Transcription activator-like (TAL) effectors specifically bind to double stranded (ds) DNA through a central domain of tandem repeats. Each TAL effector (TALE) repeat comprises 33–35 amino acids and recognizes one specific DNA base through a highly variable residue at a fixed position in the repeat. The crystal structures of TAL effector (TALE) proteins bound to their respective target DNAs have revealed that the residue at position 13 is the only one directly involved in DNA base recognition, whereas the 12th residue stabilizes the proper loop conformation. dHax3, an engineered TALE protein, proved to be a useful scaffold for structural characterizations. We then present fifteen crystal structures of engineered dHax3 variants in complex with target DNA molecules, which elucidate the structural basis for the recognition of bases adenine (A) and guanine (G) by reported or uncharacterized TALE codes.

The structural observation suggests that Ile34 may not be a major contributor to the affinity of DNA binding by TALE repeats, consistent with the classification of NI as a “weak” TALE code. It also insinuates that base A may “tolerate” a wide range of amino acids at position 34 of a TALE repeat when there is no steric clash. To test this speculation, we generated dHax3 variants with the 34th residue on repeat 7 substituted with different amino acids. In total, we obtained nine high-quality structures that elucidate the accommodation of base A by Leu, Met, Cys, Pro, Trp, His, Thr, Asn, and Glu at the 34th position. Among these, the hydrophobic residues Leu, Met, Cys, and Pro all adopt conformations that do not clash with base A. As what happens to Ile34, there is no specific coordination found between these hydrophobic residues and base A. Trp, Thr, and His, in spite of the presence of polar groups, do not form H-bond with base A. They also appear to adopt conformations that simply avoid steric clash. These residues may all represent weak code, if they are used for base recognition.

>[2x]MQWSGARALEALLTVAGELRGPPLQLDTGQLLKIAKRGGVTAVEAVHAWRNALTGAPLNLTPEQVVAIASHDGGKQALETVQRLLPVLCQAHGLTPQQVVAIASHDGGKQALETVQRLLPVLCQAHGLTPEQVVAIASHDGGKQALETVQALLPVLCQAHGLTPEQVVAIASNGGGKQALETVQRLLPVLCQAHGLTPQQVVAIASNGGGKQALETVQRLLPVLCQAHGLTPQQVVAIASNGGGKQALETVQRLLPVLCQAHGLTPQQVVAIASNPGGKQALETVQRLLPVLCQAHGLTPQQVVAIASNGGGKQALETVQRLLPVLCQAHGLTPQQVVAIASHDGGKQALETVQRLLPVLCQAHGLTPEQVVAIASNGGGKQALETVQRLLPVLCQAHGLTPEQVVAIASHDGGKQALETVQRLLPVLCQAHGLTPQQVVAIASNGGGRPALESIVAQLSRPDPALAALTNDHLVALACLGGRPALDAVKKLEHHHHHH Banna virus (BAV) is the prototype Seadornavirus, a class of reoviruses for which there has been little structural study. Here, we report atomic cryo-EM structures of three states of BAV virions—surrounded by 120 spikes (full virions), 60 spikes (partial virions), or no spikes (cores). In the full and partial BAV virions, genomic dsRNA segments and a number of RNA-dependent RNA polymerases (RdRps, VP1) are packaged in a double-layered icosahedral capsid consisting of three proteins (VP2, VP8, and VP10). The spikes protruding from the outer capsid shell are heterohexamers composed of a VP4 trimer capped by a VP9 trimer.

Visual inspection and 2D class averaging of purified BAV YN15-126-01 virions on cryo-EM micrographs revealed two types of virions: one surrounded by more spikes on the viral surface (hereafter referred to as full particles), and the other with sparser spiky density (partial particles). The ratio of full to partial particles was approximately 3:1. Icosahedral reconstructions of full and partial BAV particles (at ~5.7 Å resolution) revealed that they share overall structural features except for the different number of spikes on the virus surface. In the full BAV virions, there are 60 spikes sitting on VP10A and VP10B, respectively, while in the partial virions, there are only 60 spikes on VP10A. The binding affinity of spikes at the two channels appears different, resulting in detachment of half the spikes when the partial particles form. In the cryo-EM structure at overall 6 Å-resolution based on ~1400 acidified virus particles, 16-nm rod-shaped projections (the density of VP4 at ~15 Å local resolution) arise only from VP10A at the type II channel, suggesting that the specific shedding of spikes that occurs on partial particles may be required to form this acidified conformation. BAV entry into the cell is a highly ordered process with stepwise detachment of viral spikes, as reflected by the variation in spike arrangement on full particles (120 spikes containing VP4 and VP9), partial particles (60 spikes containing VP4 and VP9), acidified particles (60 spikes containing VP4), and core particles (no spikes).

>[2x]MPRKKDQVTKNDDGNQTSDVQTQDFKTAVQPDTNTAQLIKTYSNPKQRGDKGEIIYDGGLSSKLADVVDKTTEPHNADGAVKDGRIAPVKLDLEKQKLDKLKLFETSPFDPLTIKNNQDVVDKLYATQSSSIQEVVPTKTFATELQFGVTSEDMAKIYGAVAAVSKNVNSSVTYEVKRGTHELIKVPTIPHNLVLIQSDNGKHALIKEDLGQWPVETGISLVNQAGVFAVQLANKLGIDKPFVLDAGSNYFTDTSFIDTRKYCTDGLSPREIQKALNRQRAYYDRPELTISENKTLLSQSIIYPDADGNDVSIIFSGAMSHAIFTYAQSQWNKNIIKLDDYIREITLTVPKQYRPRRFKEIEHTHGYVYRELNQGSLLPLVDANLKESSSYYFKKLMSSISNVPVDARTLQSATAALAADTGQAVNRAQHVSMLTNRLTTANAPTVRAITVLTCMFKQFRIGMTYALDPNIMDVAAATCMLLFRPAQSISDEQYRYCLQTMAVFLTNTTYDIVNNDTIDVLKMKLRNQGWPFVERYNAVEIDMSVEPLRSPGQVGRYYNPFNIDPLTKKHVEDRLEEFINQVQVGRFRNASGNAVGTTLAAFLRACRDKTSANWRGYSVLVSRYRSLIPNELFESLRNISGEYNINPQDEHSFFFALAQINADDEFIGAIDKESAEYLDEYATLARDISNSLTLVKAAFGPLERTSGSIINHANNLNKVINHVFADKPLISETMLKILTIDGTTGKDGYRNWLDKLVGHNYPVYVEPVVNIMNFISARFVADSSYFGYTNEIMIMPNHINVPVDDRFGFRDSPFCTSLPRTIMGNDVRRISYNVFSMMEDIDDVISEGFILYDAYFNFSYDIMTTDGVTRLKEDILIVTDTGNDIKPIHFYIYFENRNDKKLRYESKMNVSYRLYIKTPACLLPLSDYMRAQHDYVSPSSSRVYIKDPAVVYTRS;>[13x]MANRATSAFLDNPHPVGVNYVDEGSRQFVAVAELLASKLIDSSRESDESNSDVPFVQAYSKFADDNPRHLRVKTGGKMANALTNVIRSYYSINAPAIVPQVEIDRLASKATVSGDMYNSYAIFNSVPIVEVLSPARTTVSIVGSDRADVTMLNTGAGAANITFNFGQIAETVILKGSVPFQLARLNQPMPAARFTYKLRPLDGPFIVVLPVGNPLVISATAATRIQVPLAFNKALVESGFQTAMNDGLFDIQNVNYYSSFDEFIISQYHAQDGINRVSTCVILGLALQAYDQMRRALPVRRV;>MDVLSKGSLKELLAHLEKTPLEEAISYRIGTVPYQNVLISRNEYYNQLYPDTTSLIDGVSREGQRNVNGLIMSIISYVVSGSGHYIPNIGFMLLRRSILDILTKHDTGLVTNNLNYGIIARNLTVSKMNCEQRKRMLICFKLLAYKDGNQNDYEIYLNQNIPLKQIAPNFIPGDMRTVIHNQDQLAIVGIPAYRLTQSTELSIRDDNAKSYKLGYVDWYNSNSFLRERSEFNLIRLKDRDTKYGKLNGW[2x];>[3x]MAWVTQAYSSGLSQNSIISLTGNDRTVADGTFNSMIMPRAVIANEREHFMKTRIDKIEHDLNRSAKQEMMDRQSLAEDYNALNLAVGQEIKLDIATQHQLNRLGSAMYKADHERETELTDLINRIRENEVTVNGILENQKAITAAERADLLLEVVASTAKSVSAAGRAAADGSGVVPVFGPSVANGIKVGIDIADSVAEAAIAVKESGIITQLNDVYHAFQSVHVAPNDVIKPAAVVAGTSTELIGNLQAIYSRLRSHSDIGFKKATVGDVIPNSYMIKPVNSTEYASWQLYVIHPVQGSLGLVVQLMGDALTYNVFAQYGNTSASEFGKTVLTGGATNTALEGTKVKFQTKVTAQQALALTMALKDAASMLSQGELIGYFEQYINLALEPDNLSLQDNMHKYHHLLTSQNSPIDWNYHDEEMHKWLDSRKTTNYDAMQKKDGTVIADIHIPKVFNDLRNTTLHCKLEGKQTIAGYTVYEYLIGPWAHYGDIDYSVVVDTLNEETKWYCEVIGIDGHLLIEKSVQHKPEKILELTVNDSGVTSFNGRNHDRLKLKVYVKDSLSVKVFRNWIGINAPRVKTKMFNDHIGVKYDYSHFDKNISPAHLTLTDLGWHTWDQYNAGNWTNIKP;>MLSETELRALKKLSTTTSRVVGDSTLALPSNVKLSKGEVEKIAVTKKEMFDELAQCNLPTIELITREHTFNGDVIRFAAWLFLMNGQKLMIANNVAVRMGMQYATNLAGNNVKITYVTSNNVVKLGHIAAGVLANPYSNKGSGLFITYEYNLISNLIETGKVCVLFITSLSTTASSTNSFAYSTCSVPIENWDFNMIKLTAETSCASLTAMTNLVNSLVPGERTRPVGLYVDIPGVTVTTSASSGSLPLTTIPAVTPLIFSAYTKQVEEVGVINTLYALSYLP[3x]> GSSH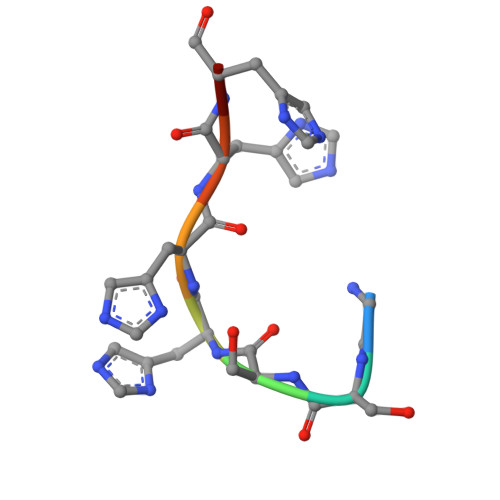HHHH> GLTYCTHASGFSFNPQTADAGTSMNVVTEQIYNKLFDIKNHSATLTPMLAQSYSISADGKEILLNLRHGVKFHQTPWFTPTRDFNAEDVVFSINRVLGHNTYLPTLAEANVTYSNPQYKVFHEQARKVRFPYFDSIKLNEKIKSVTALSPYQVKIELFAPDSSILSHLASQYAIIFSQEYAYQLSADDNLAQLDTHPVGTGPYQVKDYVYNQYVRLVRNENYW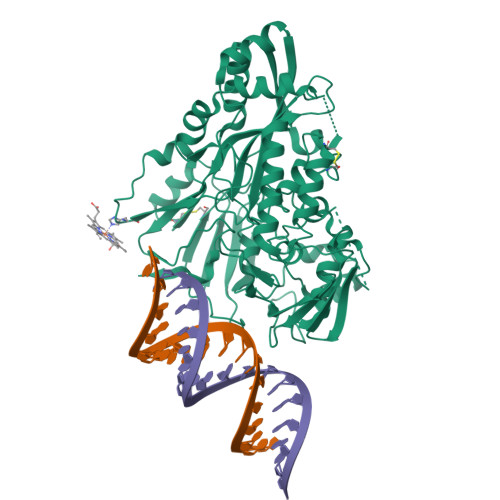KKEAKIEHIIVDLSTDRSGRLVKFFNNECQIASYPEVSQIGLLKNDDKHYYMQSTDGMNLAYLAFNFDKPLMRDHEIRAAISQSLNRARIIHSIYHNTATVANNIIPEVSWASTVNTPEFEFDYHPKIAKNKLADKNLLLNLWVINEEQVYNPAPFKMAEMIKWDLAQAGVKVKVRAVTRPFLTAQLRNQLENYDLILSGWLAGNLDPDGFMRPILSCGTKNELTNLSNWCNEEFDQFMDRAITTSHLSSRAKAYNEAQELVLRELPIIPIANVKRILVANSRVKGVKMTPFGSLDFSTLYFI>[2x]S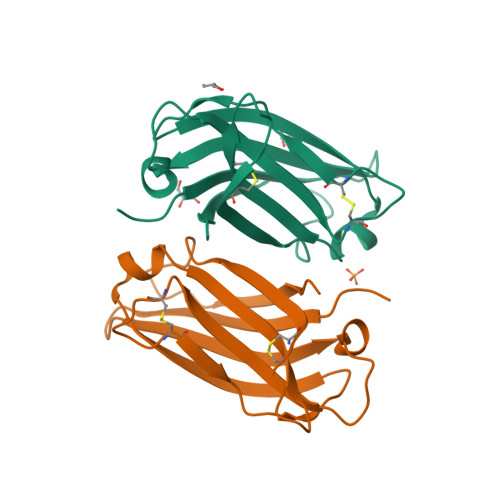GATRIQIALKYDEKNKQFAILIIQLSNLSALLQQQDQKVNIRVAVLPCSESTTCLFRTRPLDASDTLVFNEVFWVSMSYPALHQKTLRVDVCTTDRSHLEECLGGAQISLAEVARSGERSTRWYNLLS> SDRAEVRNIPFKLGMYLTVGGVVNSNATRFSINVGESTDSIAMH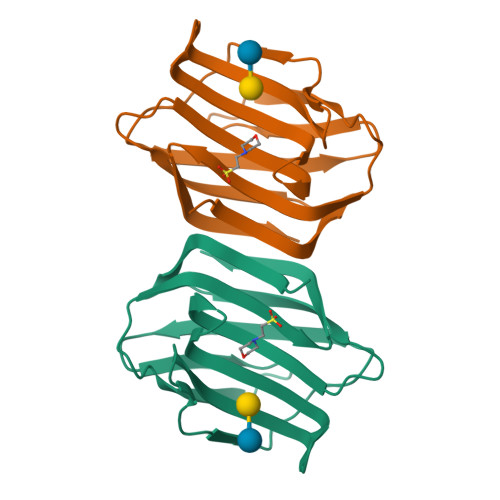MDHRFSYGADQNVLVLNSLVHNVGWQQEERSKKFPFTKGDHFQITITFDTHTFYIQLSNGETVEFPNRNKDAAFNLIYLAGDARLTFVRLE> MEIVEYPDPILRAKNKRIDIFDENLKNLVDAMFDVMYKTDGIGLSAPQVGLNVQLMVFNPAGEPGEGKEIVLVNPKIKKYSDKLVPFDEGCLSFPGIYAEVVRPQSVKIDARDITGERFSISLSRLPARIFQHEYDHLEGVLFFDRMTDQVLDSIREELEALEKKYEEKTGLPSPERVEARQKRKAGVGFGKR

Here, we explore the precise structural inhibitory mechanism of actinonin, which is a slow, tight-binding inhibitor of peptide deformylase (PDF), a metal cation-dependent enzyme. PDF is the first enzyme in the N-terminal methionine excision pathway, an essential and ubiquitous process that contributes to the diversity of N-terminal amino acids. The function of the active-site metal is to activate the reactive water molecule involved in peptide hydrolysis. Actinonin is a natural product with antibiotic activity that inhibits PDF by mimicking the structure of its natural substrates (nascent peptide chains starting with Fo-Met-Aaa, where Fo is a formyl group and Aaa is any amino acid) in their transition state.

In this respect, we studied the binding of compound 6b, a PDF ligand that does not exhibit a reactive group at this position. We observed that this compound binds strongly to both EcPDF (KI*  = 63±6 nM) and AtPDF (KI*  = 400±35 nM) but, unlike actinonin, does not display slow, tight binding as KI*  =  KI. This impact on binding is consistent with the absence of the hydrogen bond involving the first carbonyl group of the ligand. The 3D structure of AtPDF was determined after soaking the compound in crystals of the free, open AtPDF form. Upon binding, 6b induced a complete conformational change, identical to that observed with actinonin (“O” state). This result further suggests that the conformational change is not induced initially by the formation of this hydrogen bond and that the encounter complex is primarily driven by the fit within the S1' pocket. The 3D structure also revealed that both the P1' and the hydroxamate groups are bound similarly to the corresponding groups of actinonin. As expected, no additional bonding occurs, especially around the backbone nitrogen of Ile42. Taken together, these data allow us to conclude that the conformational change observed upon ligand binding is triggered primarily by binding in the S1' pocket. As revealed by the binding of 6b, the one carbon longer metal-binding group fits, immediately upon recognition of the P1' group, in the S1' pocket and forms a bidentate complex with the metal cation, mimicking the transition state as a result.>[4x]MNRLQHIRGHIVSA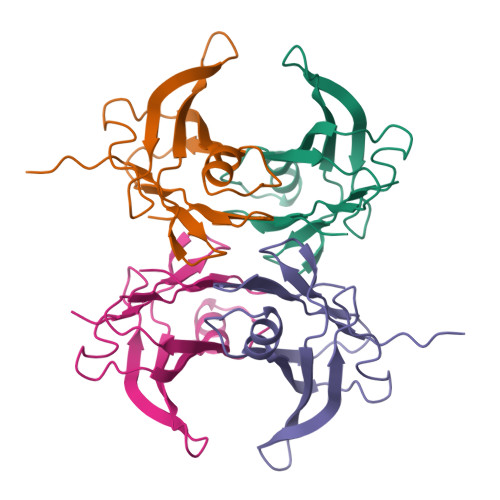DKHINMSATLLSPLSTHVLNIAQGVPGANMTIVLHRLDPVSSAWNILTTGITNDDGRCPGLITKENFIAGVYKMRFETGKYWDALGETCFYPYVEIVFTITNTSQHYHVPLLLSRFSYSTTRGS>MTAHDLIDEIIQDVIQLDGKLGLLGGNTRQLEDGRVINIPNGAAMIFDDYKKYKQGELTAESALESMIKIAKLSNQLNRHTFFNQRQPETGQFYKKVAAIDLQTTIAAEYDNNHGLRILE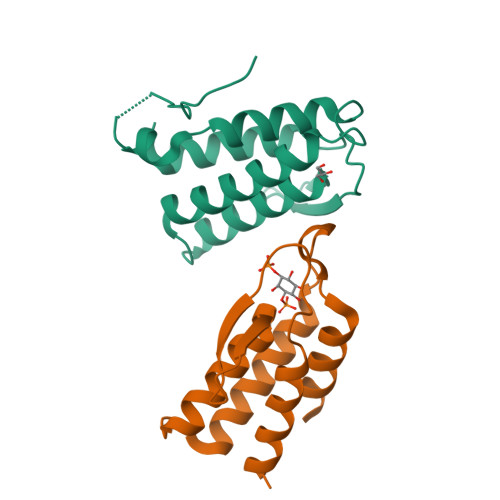HHHHHH[2x]>[2x]G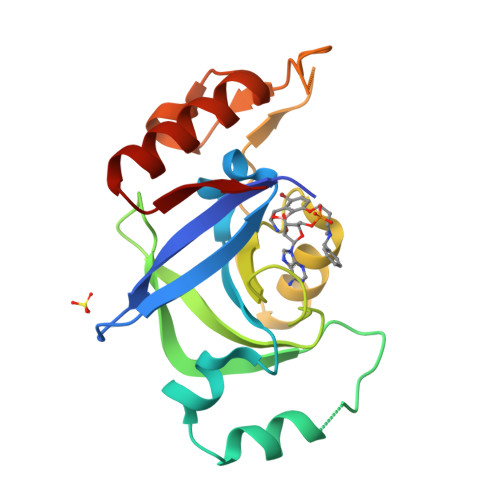AMGKSEGVTIEFKIVGLNKKLKVFTTCPHTLFGASFCAVAIEHPIVQDLMSKEIQDLISSIKIQGKNNEKVGIYTGLNVKHPFLDKELPLYVANFVLMEYREGAIFGCPAHDQRDFEFAQEYDLPIIPVISSARLGIEEYTNNSIMFNSEFLNGLTVSEARKVIVEKLEEKGIGKKTI>[4x]TPPNAPVVTYSDIVNDLIIMQGTAEAKSQLIITDSEGNTYTLTVPDNGKWSMAIPYPSEGKFTIT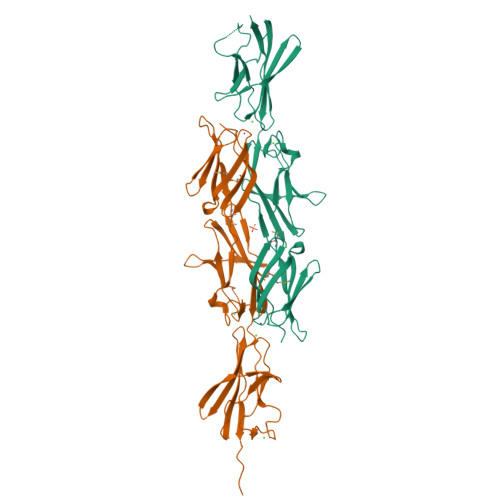SVDAIGNRSDDVPLDIMKEVPVISLSPDSDSGTVGDNITRDKQPTFIIGNLESDVVVVQVDINGTVYNAEKNADGVWFFTPGTPLADGSYTISVIASDAAGNQKNSLPITVTIDSTLTVPEIALAAGEDNGASDSDNVTNHTQPKFTLQHIDADVTGVTVNVTHNGVTDIYQATQGADGWTFTPPAAWNDGNYTLSVTVVDRAGNSQQSASLAVTVDSTVTVT>MPARRPFIGGNFKCNGSLDFIKSHVAAIAAHKIPDSVDVVIAPSAVHLSTAIAANTSKQLRIAAQNVYLEGNGAWTGETSVEMLQDMGLKHVIVGHSERRRIMGETDEQSAKKAKRALEKGMTVIFCVGETLDERKANRTMEVNIAQLEALGKELGESKMLWKEVVIAYEPVWSIGTGVVATPEQAEEVHVGLRKWFAEKVAAEGAQHIRIIYGGSANGSNDEKLGQCPNIDGFLVGGASLKPEFMTMIDILTKT[20x]

TIM is a ubiquitous glycolytic enzyme whose active site and overall α8/β8 barrel domain structure are highly conserved; even so, structural differences in its interface region have been used to achieve specific inhibition of enzymes in parasites. Since Giardia lacks oxidative phosphorylation and depends on glycolysis as its major ATP source, it has been proposed that disrupting this pathway could hinder the survival of the parasite; therefore, glycolytic enzymes have been considered potential pharmacological targets. Our results indicated that derivatization of C222, a non-interfacial residue located near the surface of the protein and 10-15 Å away from the active site, specifically inactivates the enzyme. C222 is at the end of loop 7, with its lateral chain positioned in a hydrophobic pocket formed mainly by carbon atoms of residues N218, G219, E223, F234, M248, and I251.

C222N and C222D respectively exhibited a catalytic efficiency 10-fold and 17-fold lower than that of WT GlTIM, indicating that electrostatic factors in the region of C222 are central in the expression of catalytic activity of GlTIM. The most severe changes in the Ki values were when negatively and positively charged residues were introduced; for the C222D mutant, an 83-fold increase in the Ki was observed. On the other hand, the C222DC mutant produced triclinic crystals with a P1 symmetry that contains 10 dimers per asymmetric unit. WTC and C222NC produced high-resolution structures (1.6Å and 1.45Å, respectively), whereas C222DC was solved at a resolution of 2.7Å. The C222DC structure had an empty active site, which is consistent with the binding data that indicate the low affinity of C222D for 2-PG. The crystal structure of C222DC provided a clear atomic description of the structural changes induced by modification of C222 that explain the observed detrimental effects on GlTIM. In this structure, it is relevant that the 20 monomers of the asymmetric unit display structural variations in two specific and localized regions of the protein. The structural alignment of all monomers showed that loop 6 (residues 175 to 182) and loop 7 (residues 214 to 221) exhibit a clear heterogeneity of conformational states, which is evidenced in the per residue α-carbon RMSD values of all chains. In regard to loop 7 it is important to highlight that even though slight conformational changes in this loop had been previously noted in response to ligand binding, the relatively large conformational differences of loop 7 in the C222DC structure has not been previously observed; its main chain atoms move as far as 2.7 Å from their original position. Therefore, it is reasonable to assume that the introduction of a negatively charged side chain in the low dielectric environment of this hydrophobic pocket is a thermodynamically unfavorable process that destabilizes the entire loop 7, and alters the structure of the critical YGGS motif.> SYHPKPWLGAQPATVVTPGVNVTLRCRAPQPAWRFGLFKPGEIAPLLFRDVSSELAEFFLEEVTPAQGGSYRCCYRRPDWGPGVWSQPSDVLELLVTEELPRPSLVALP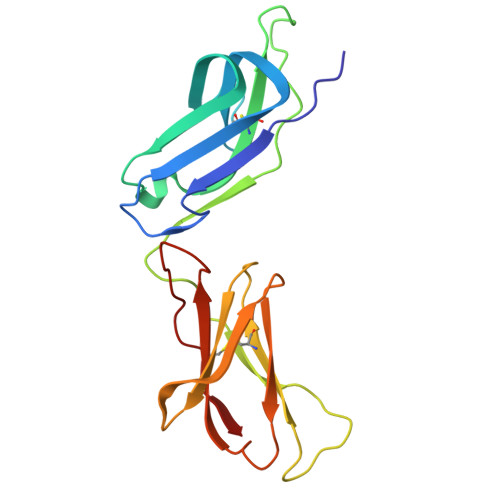GPVVGPGANVSLRCAGRLRNMSFVLYREGVAAPLQYRHSAQPWADFTLLGARAPGTYSCYYHTPSAPYVLSQRSEVLVI> LASVIPDVATLNSLFNQIKNESCGTSTASSPCITFRYPVDGCYARAHKMRQILMNNG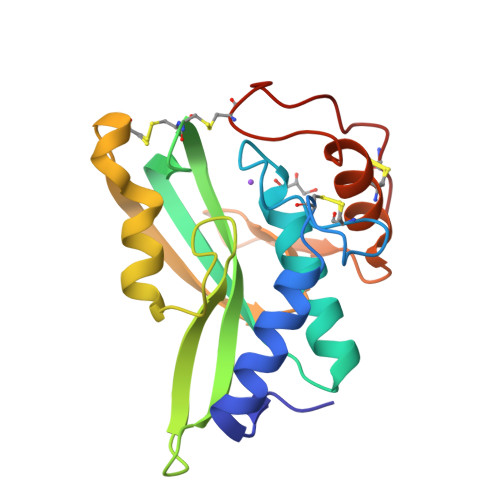YDCEKQFVYGNLKASTGTCCVAWSYHVAILVSYKNASGVTEKRIIDPSLFSSGPVTDTAWRNACVNTSCGSASVSSYANTAGNVYYRSPSNSYLYDNNLINTNCVLTKFSLLSGCSPSPAPDVSSCGF> GDDTKTYILSLPNYETHTLDMGDQENPDDSWSVSSEWGTTNYKYNLLTDASGIFEFDCVSSTYGFYSDSFAFTNCTVEDCPDFASYDYRAITKKGVINNTYVIVGAAGYKIGKNSDKEAAIRFRDHDNPNELEDYRVKGLYVTNSVYAYSSMKEGTGYYGEEEIFGSNDSFKLTIYNYDKTMHVDCYLAEGTNLLD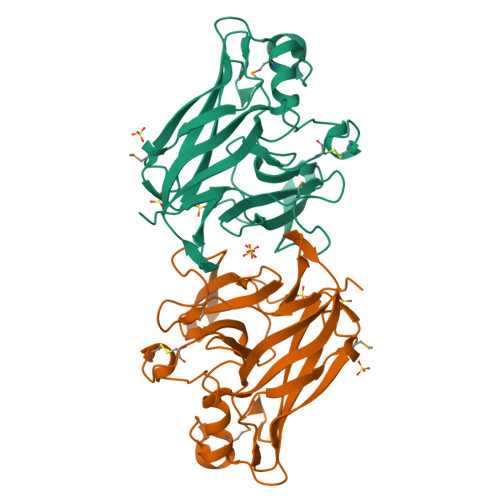QWKWVDLTSLGETKGLKFSLTSTKKNEYGPLTPTYFCLDGITIED1-(3-fluorophenyl)-N-[trans-4-(2-hydroxypropan-2-yl)cyclohexyl]-1,4,6,7-tetrahydro-5H-pyrazolo[4,3-c]pyridine-5-carboxamide 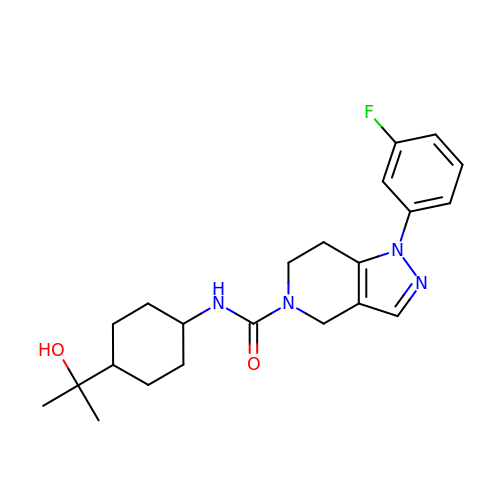| C22 H29 F N4 O2 | APPNXGOPROLJQR-SAABIXHNSA-N>MSGKLTVITGPMYSGKTTELLSFVEIYKLGKKKVAVFKPKIDSRYHSTMIVSHSGNGVEAHVIERPEEMRKYIEEDTRGVFIDEVQFFNPSLFEVVKDLLDRGIDVFCAGLDLTHKQNPFETTALLLSLADTVIKKKAVCHRCGEYNATLTLKVAGGEEEIDVGGQEKYIAVCRDCYN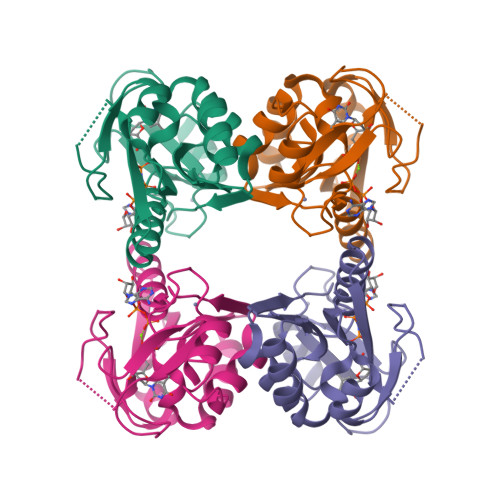TLKKRV[2x]KANAMYCIN A | 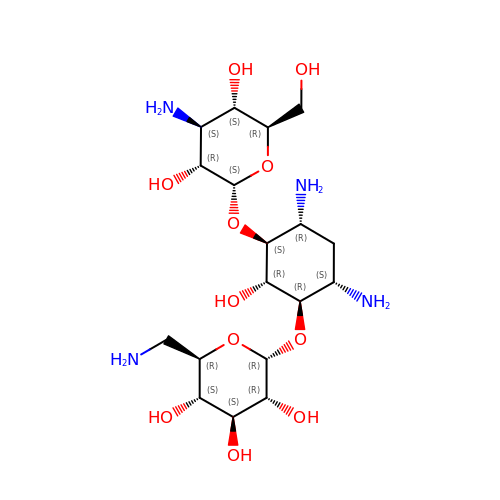C18 H36 N4 O11 | SBUJHOSQTJFQJX-NOAMYHISSA-N> HPETLVKVKDAEDQLGARVGYIELDLNSGKILESFRPEERFPMMSTFKVLLCGAVLSRVDAGQEQLGRRIHYSQNDLVEYSPVTEKHLTDGMTVRELCSAAITMGDNTAANLLLTTIGGPKELTAFLHNMGDHVTRLDRWE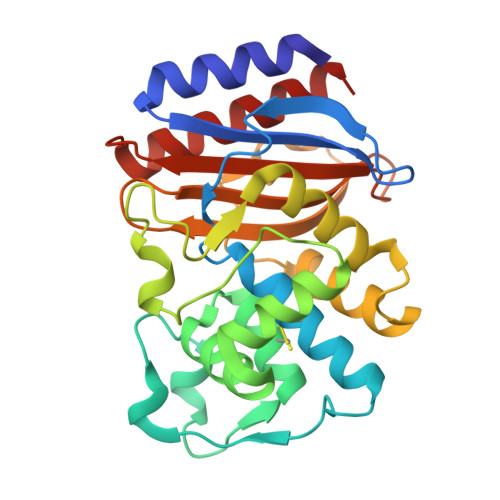PELNEAIPNDERDTTMPAAMATTLRKLLTGELLTLASRQQLIDWMEADKVAGPLLRSALPAGWFIADKSGAGERGSRGIIAALGPDGKPSRIVVIYTTGSQATMDERNRQIAEIGASLIKHW> MKKQKRTQGKQNTKQIKQEKLSSKRKANNQKEGKKKVKQEDYKEIKQKGKRMLSKIVKASFSSKGFNLANAVNTVKSTLNAPIKHIKRNIEPTGSNYSRMTNTTEEAFDEVSHEWQALVTSNPFDLNVFNYLENTQTSNFGTVDNPLVVFTSETPFRYVGCTGQMNEDDYEGHELLFFLLREGSLQRCMGCGQVFKLVRLRNEYSPEMDYYLSNFHPYEMQEMGESDTTVLMSPYKYASHYEYTQFETPSNMVYSMVNPDEHDRLLVDPAYRMERTKALEEKYKVYTSSLREVEKQFEERYGRAGQINISKVTYSTLIDVEKAVLKMDRLFRKVAKFENRAFIDRANHSRREKRMLERAQQRWDSNYSFFTGSLTEEEQKYRDYYETELEAYPEDEGIEQQLDQQEVLLSGRYDPKLYDFQ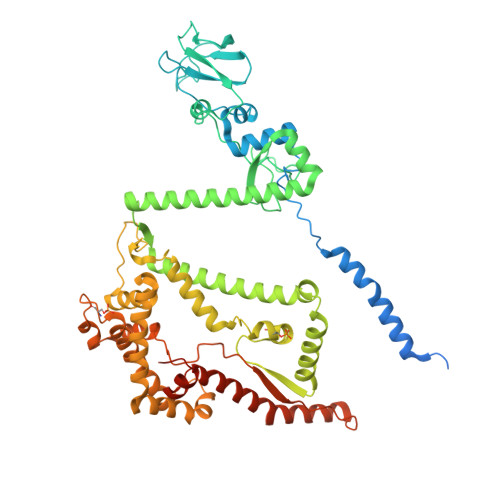EGYTKNPEDDQTSLIEKKAFKFRYRLANETSETFQRRNNRMVERQIKRFQQPQYKHAFEQLQKNIAISSNSGNALHSEYGYLELLSNESVQLYKDYYESDAEEDFKVFENLSSKEKLVMIANFENNLLPKYDRSEVHLIPKRQWEPAFGVWENFLYDITEYASFIAPRGKEIAADYQIQSAIPLTKEELIEAGLYKETIEKKVEPKLEAKKQTKSE>TMAASQTSQTVASHVPFADLCSTLERIQKSKGRAEKIRHFREFLDSWRKFHDALHKNHKDVTDSFYPAMRLILPQLERERMAYGIKETMLAKLYIELLNLPRDGKDALKLLNYRTPTGTHGDAGDFAMIAYFVLKPRCLQKGSLTIQQVNDLLDSIASNNSAKRKDLIKKSLLQLITQSSALEQKWLIRMIIKDLKLGVSQQTIFSVFHNDAAELHNVTTDLEKVCRQLHDPSVGLSDISITLFSAFKPMLAAIADIEHIEKDMKHQSFYIETKLDGERMQMHKDGDVYKYFSRNGYNYTDQFGASPTEGSLTPFIHNAFKADIQICILDGEMMAYNPNTQTFMQKGTKFDIKRMVEDSDLQTCYCVFDVLMVNNKKLGHETLRKRYEILSSIFTPIPGRIEIVQKTQAHTKNEVIDALNEAIDKREEGIMVKQPLSIYKPDKRGEGWLKIKPEYVSGLMDELDILIVGGYWGKGSRGGMMSHFLCAVAEKPPPGEKPSVFHTLSRVGSGCTMKELYDLGLKLAKYWKPFHRKAPPSSILCGTEKPEVYIEPCNSVIVQIKAAEIVPSDMYKTGCTLRFPRIEKIRDDKEWHECMTLDDLEQLRGKASGK[2x]

DNA ligase IV (LigIV), one of three DNA ligases in higher eukaryotes, plays a central role in the repair of DNA double-strand breaks (DSBs) during nonhomologous end joining (NHEJ). Human DNA ligases have a conserved catalytic region consisting of a DNA-binding domain (DBD), a nucleotidyltransferase domain (NTD), and an OB-fold domain (OBD) (Tomkinson et al., 2006). A covalent AMP-lysine intermediate is formed with the catalytic lysine (K273) in motif I of LigIV (step 1) before the AMP is transferred to the 5′ phosphate of the DNA nick (step 2). Artemis is activated by the autophosphorylation of DNA-PKcs (Goodarzi et al., 2006). It has recently been found that Artemis (residues 485–495) also interacts with LigIV (Malu et al., 2012).

We also solved the structure of LigIV1–609 without Artemis485–495 at 2.84 Å resolution. The structures proved to be very similar except for the conformation of the loop between β11 and β12, which is distorted by the binding of thiomersal in the mercury derivative (data not shown). After we submitted our manuscript, De Ioannes et al. reported the structure of DBD of LigIV in complex with Artemis485–495 (De Ioannes et al., 2012). Comparison of the two structures indicates very similar interactions between LigIV and Artemis (the root-mean-square deviation [rmsd] of Cα atoms of the structures is 0.975 Å calculated using LSQKAB in CCP4; Kabsch, 1976). However, the rmsd of their and our structures without Artemis is 6.88 Å, which is mainly a consequence of a difference in the conformations of α2 and the region after α10. However, the conformations of α2 with and without Artemis485–495 in our structures are very similar. The difference between the two studies is probably due to the presence in our structure of NTD, which stabilizes the conformation of the region after α10 via contacts with α11, the following loop and that connecting α12 and NTD. α2 interacts with this region and its conformation is likely affected by it. In the crystals, the structure of LigIV1–609 is captured in an open conformation and probably stabilized by burying a surface of area 1,104 Å2 between OBD and NTD. In nonderivative crystals, the electron density of adenosine is clearer in the catalytic pocket of LigIV1–609 molecules. In addition, extra density near the adenosine is not explained by fitting AMP molecules, indicating that ATP may bind to LigIV1–609 molecules that are not adenylated.>AAESGVSRPVPQLKRTTMRILIGLLVQNPELATLVPPLENLDENKLPGLGLFRELVNTCLSQPGLTTGQLLEHYRGTNNAATLEKLSMWDDIADKNIAEQTFTDSLNHMFDSLLELRQEELIARERTHGLSNEERLELWTLNQELAKKTRESGSIGSMDFDDDI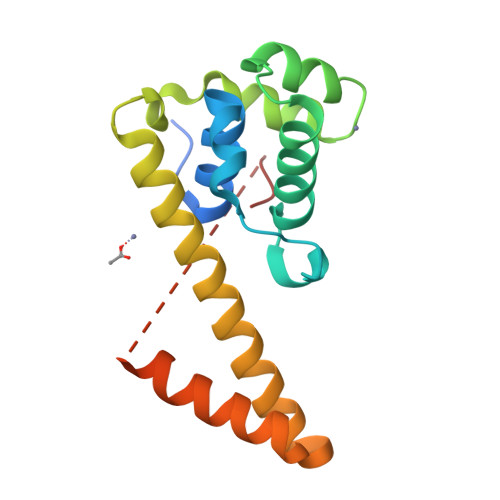PF[2x]6,7-dimethoxy-~{N}-[(1~{R})-1-phenylethyl]quinazolin-4-amine | C18 H19 N3 O2 | 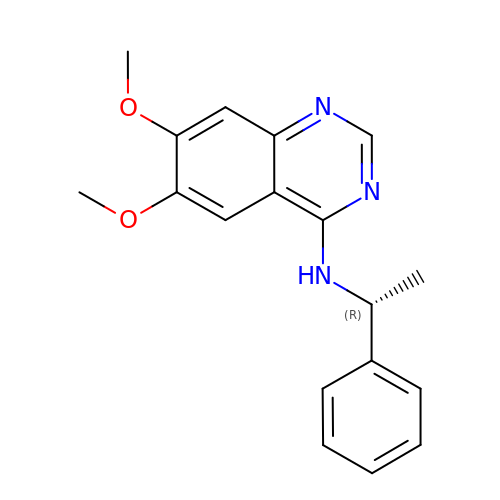RJFMUYZWDLSYSX-GFCCVEGCSA-N>AALGVQSINWQTAFNRQAHHTDKFSSQELILRRGQNFQVLMIMNKGLGSNERLEFIVSTGPYPSESAMTKAVFPLSNGSSGGWSAVLQASNGNTLTISISSPASAPIGRYTMALQIFSQGGISSVKLGTFILLFNPWLNVDSVFMGNHAEREEYVQEDAGIIFVGSTNRIGMIGWNFGQFEEDILSICLSILDRSLNFRRDAATDVASRNDPKYVGRVLSAMINSNDDNGVLAGNW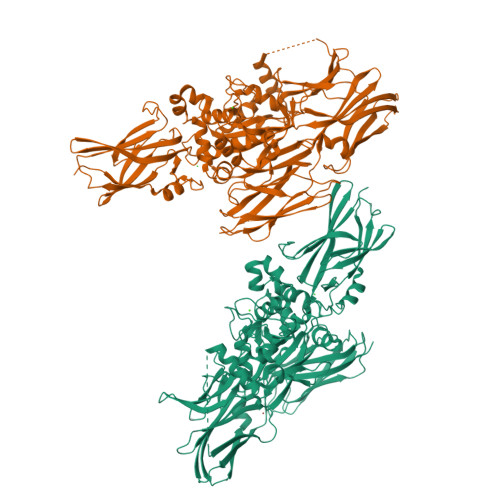SGTYTGGRDPRSWDGSVEILKNWKKSGLSPVRYGQCWVFAGTLNTALRSLGIPSRVITNFNSAHDTDRNLSVDVYYDPMGNPLDKGSDSVWNFHVWNEGWFVRSDLGPSYGGWQVLDATPQERSQGVFQCGPASVIGVREGDVQLNFDMPFIFAEVNADRITWLYDNTTGKQWKNSVNSHTIGRYISTKAVGSNARMDVTDKYKYPEGSDQERQVFQKALGKLKPNTPFAATSSMGLETEEQEPSIIGKLKVAGMLAVGKEVNLVLLLKNLSRDTKTVTVNMTAWTIIYNGTLVHEVWKDSATMSLDPEEEAEHPIKISYAQYERYLKSDNMIRITAVCKVPDESEVVVERDIILDNPTLTLEVLNEARVRKPVNVQMLFSNPLDEPVRDCVLMVEGSGLLLGNLKIDVPTLGPKERSRVRFDILPSRSGTKQLLADFSCNKFPAIKAMLSIDVAE[2x]Banna virus (BAV) is the prototype Seadornavirus, a class of reoviruses for which there has been little structural study. Here, we report atomic cryo-EM structures of three states of BAV virions—surrounded by 120 spikes (full virions), 60 spikes (partial virions), or no spikes (cores). In the full and partial BAV virions, genomic dsRNA segments and a number of RNA-dependent RNA polymerases (RdRps, VP1) are packaged in a double-layered icosahedral capsid consisting of three proteins (VP2, VP8, and VP10). The spikes protruding from the outer capsid shell are heterohexamers composed of a VP4 trimer capped by a VP9 trimer.

Immediately inside the inner capsid, RdRp is located near the fivefold vertices. Asymmetrical reconstruction focused on icosahedral vertices revealed clear density for a non-transcribing RdRp (VP1) molecule near the fivefold pore within the inner capsid shell, and nearby dsRNA is also visible at low contour levels. Compared with adjacent VP2 subunits in the inner capsid, VP1 shows increased B-factors. Like other reported reovirus RdRps, the N-terminal domain and C-terminal “bracelet” domain cover the BAV RdRp “fingers–palm–thumb core”, forming a cage-like structure with four channels connected to the reaction center. Only one N-terminal tail of a VP2A subunit interacts with the C-terminal bracelet domain of RdRp, near the C5 exit channel, suggesting that BAV RdRp may be less stable within the inner shell compared with other sedoreovirus RdRps.

>MPRKKDQVTKNDDGNQTSDVQTQDFKTAVQPDTNTAQLIKTYSNPKQRGDKGEIIYDGGLSSKLADVVDKTTEPHNADGAVKDGRIAPVKLDLEKQKLDKLKLFETSPFDPLTIKNNQDVVDKLYATQSSSIQEVVPTKTFATELQFGVTSEDMAKIYGAVAAVSKNVNSSVTYEVKRGTHELIKVPTIPHNLVLIQSDNGKHALIKEDLGQWPVETGISLVNQAGVFAVQLANKLGIDKPFVLDAGSNYFTDTSFIDTRKYCTDGLSPREIQKALNRQRAYYDRPELTISENKTLLSQSIIYPDADGNDVSIIFSGAMSHAIFTYAQSQWNKNIIKLDDYIREITLTVPKQYRPRRFKEIEHTHGYVYRELNQGSLLPLVDANLKESSSYYFKKLMSSISNVPVDARTLQSATAALAADTGQAVNRAQHVSMLTNRLTTANAPTVRAITVLTCMFKQFRIGMTYALDPNIMDVAAATCMLLFRPAQSISDEQYRYCLQTMAVFLTNTTYDIVNNDTIDVLKMKLRNQGWPFVERYNAVEIDMSVEPLRSPGQVGRYYNPFNIDPLTKKHVEDRLEEFINQVQVGRFRNASGNAVGTTLAAFLRACRDKTSANWRGYSVLVSRYRSLIPNELFESLRNISGEYNINPQDEHSFFFALAQINADDEFIGAIDKESAEYLDEYATLARDISNSLTLVKAAFGPLERTSGSIINHANNLNKVINHVFADKPLISETMLKILTIDGTTGKDGYRNWLDKLVGHNYPVYVEPVVNIMNFISARFVADSSYFGYTNEIMIMPNHINVPVDDRFGFRDSPFCTSLPRTIMGNDVRRISYNVFSMMEDIDDVISEGFILYDAYFNFSYDIMTTDGVTRLKEDILIVTDTGNDIKPIHFYIYFENRNDKKLRYESKMNVSYRLYIKTPACLLPLSDYMRAQHDYVSPSSSRVYIKDPAVVYTRS[11x];> MDVQEQFEGYLREEVDLLNKFEDSHFKQLEIFYTKSQTDHVINKDKLQFNALPFHTTLYKEINGKRVRLGTLLNWTKAERLDTIRHESMIKDERLRRLIDFDYGWIDYAVVLQRYLDEGNTIESANILQFDGDFVNNIKHPTQKNNFLDIKVIKECETYILMKDDNGIRDPDILRAWELNSIPEVIELDVDGETKKFNLRKEMIKRIQDEAPVYFFCNPYRYAVANLDPNIPEVRLWLEYFIGSEDFFGFNGPNVIVSKSLLAAKRFEVVVNHLRKVAAFELDVESKEVMNEWIKYIMIDPVYRSYKNRGAFGNLNQHVFARTKSEGLSWSLIDIGTTNFELKPTKKVAGSYVNKFNLVDDVLVEESLKDLRNEGLHKMADVTRRMIDADITPENVKKGKLNRLALSYCGYTGSHSATAMVKQFNGTKDLDPNCDPMFVDIVKDNMRVYMQEGLQKYPQGSRKSNRLDILFKGGTSSASSTNEHAVVNGRFRYRSELYRERDVNSSTVFKTATPGQYRVVKKISAKLKSKNANIVTHPMNFINFKVDDLDIVVNAGSRLVRGTRAKRIITPNYGTIYAASLMTVLPAVRLLSSRASNMGALSTQGRIGTTYHGALPHDVMAPQLAVTSSDDVSKICVAKDFGQFDTSQWGQISKAHADGVRSMKAHYSMGHDTLVDLDLNDASFADLLEVTAMSYERPLKYKMNGLVCESAGVKSGELTTQTRNTTTNISHSTVALDDYNNRAYRLNLPKLELVTDNKVGDDSVEVLRVVDGSPLTPEIAKLYVNCMQDHADKNHLEISAKRTIVGNNVAEHIKIWVFKGYLALDVFLDSVTSEKNSFSNLNYLEQVNILYDMAMTLMIRYCSVQACMTQFCNDMKLLNGIRAGNYTFIPTPKIICAYGTPEICLRAPEIRSFGRYLPIDEDEYSVLNDLVASLSTNKPKMDFVAQMFEQNGNQVHGIWLDHFKRKNDVNPDGGGIHISEGLKRLMPEYCERHLNELVYKTLDDKVIRDYTSDIIITNICKGKLSKAPKLAFFANFYLSLTGFNGVDSPYLTADEGVKNVHRVIGLSYRNTLSTSPTANVDRILRNNPGSAPAYLTGNDILGVLSDYPYQNWRTVVELLDITEPSATAIIEVATNQMHAYLADKDLNTANLFDNTSRTYDISDRTYPKFVNITSNLSNSNRRGFQLEAMKHIIYMARRGIATLANTHPSKIGNTVYYDY>AFELPPLPYAHDALQPHISKETLEFHHDKHHNTYVVNLNNLVPGTEFEGKTLEEIVKTSSGGIFNNAAQVWNHTFYWNCLSPNAGGQPTGALADAINAAFGSFDKFKEEFTKTSVGTFGSGWGWLVKKADGSLALASTIGAGCPLTIGDTPLLTCDVWEHAYYIDYRNLRPKYVEAFWNLV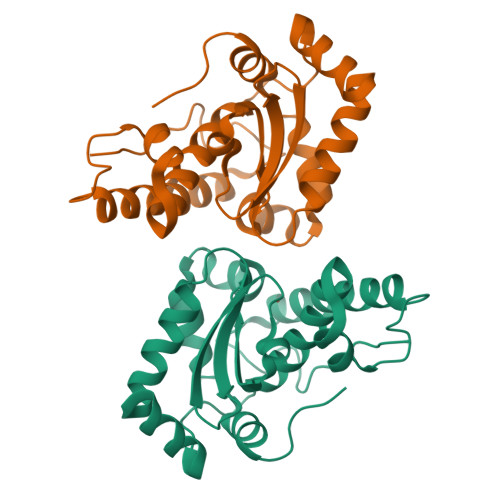NWAFVAEQFEGKTYKV[3x]>MSPTIPTTQKAVIFETNGGPLEYKDIPVPKPKSNELLINVKYSGVCHTDLHAWKGDWPLDNKLPLVGGHEGAGVVVAYGENVTGWEIGDYAGIKWLNGSCLNCEYCIQGAESSCAKADLSGFTHDGSFQQYATADATQAARIPKEADLAEVAPILCAGITVYKALKTADLRIGQWVAISGAGGGLGSLAVQYAKALGLRVLGIDGGADKGEFVKSLGAEVFVDFTKTKDVVAEVQKLTNGGPHGVINVSVSPHAINQSVQY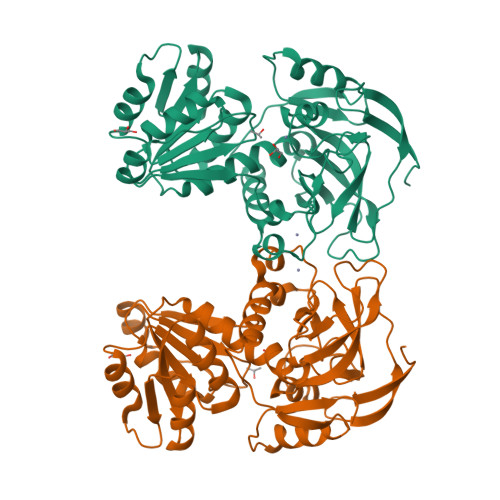VRTLGKVVLVGLPSGAVVNSDVFWHVLKSIEIKGSYVGNREDSAEAIDLFTRGLVKAPIKIIGLSELAKVYEQMEAGAIIGRYVVDTSK[2x]> DETKALKELYGPVDPTFLHRFYSLKAAVHGWKMVVCDKVRSLKLSDNNCYLNAVIMTLDLLKDIKFVIPALQHAFMKHKGGDSTDFIALIMAYGNCTFGAPDDASRLLHTVLAKAELCCSARMVWREWCNVCGIKDVVLQGLKACCYVGVQTVEDLRARMTYVCQCGGERHRQLVEHTTPWLLLSGTPNEKLVTTSTAPDFVAFNVFQGIET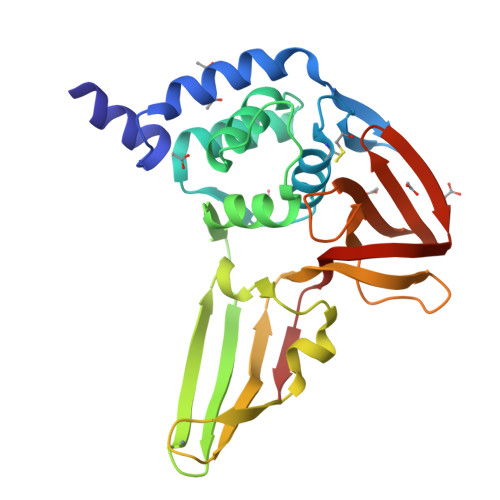AVGHYVHARLKGGLILKFDSGTVSKTSDWKCKVTDVLFPGQKYSS> MVPISPIETVPVKLKPGMDGPKVKQWPLTEEKIKALVEICTEMEKEGKISKIGPENPYNTPVFAIKKKDSTKWRKLVDFRELNKRTQDFWEVQLGIPHPAGLKQKKSVTVLDVGDAYFSVPLDKDFRKYTAFTIPSINNETPGIRYQYNVLPMGWKGSPAIFQCSMTKILEPFRKQNPDIVIYQYMDDLYVGSDLEIGQHRTKIEELRQHLLRWGFTTPDKKHQKEPPFLWMGYELHPDKWTVQPIVLPEKDSWTVNDIQKLVGKLNWASQIYAGIKVRQLCKLLRGTKALTEVVPLTEEAELELAENREILKEPVHGVYYDPSKDLIAEIQKQGQGQWTYQIYQEPFKNLKTGKYARMKGAHTNDVKQLTEAVQKIATESIVIWGKTPKFKLPIQKETWEAWWTEYWQATWIPEWEFVNTPPLVKLWYQLEKEPIIGAETFYVDGAANRETKLGKAGYVTDRGRQKVVPLTDTTNQKTELQAIHLALQDSGLEVNIVTDSQYALGIIQAQPDKSESELVSQIIEQLIKKEKVYLAWVPAHKGIGGNEQVDKLVSAGIRKVL;> MGHHHHHHMVPISPIETVPVKLKPGMDGPKVKQWPLTEEKIKALVEICTEMEKEGKISKIGPENPYNTPVFAIKKKDSTKWRKLVDFRELNKRTQDFWEVQLGIPHPAGLKQKKSVTVLDVGDAYFSVPLDKDFRKYTAFTIPSINNETPGIRYQYNVLPQGWKGSPAIFQCSMTKILEPFRKQNPDIVIYQYMDDLYVGSDLEIGQHRTKIEELRQHLLRWGFITPDKKHQKEPPFLWMGYELHPDKWTVQPIVLPEKDSWTVNDIQKLVGKLNWASQIYAGIKVRQLCKLLRGTKAL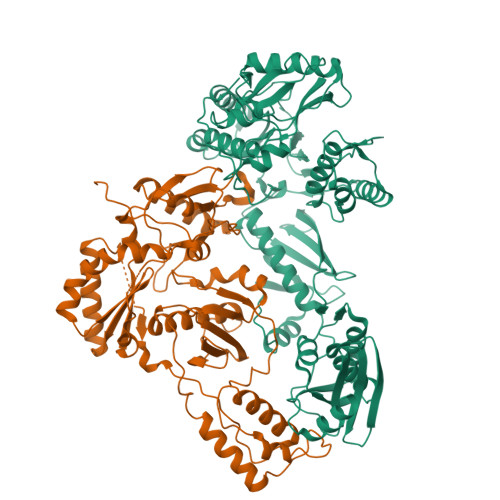TEVVPLTEEAELELAENREILKEPVHGVYYDPSKDLIAEIQKQGQGQWTYQIYQEPFKNLKTGKYARMKGAHTNDVKQLTEAVQKIATESIVIWGKTPKFKLPIQKETWEAWWTEYWQATWIPEWEFVNTPPLVKLWYQ> GDLADRFAELERRYDARLGVYVPATGTTAAIEYRADERFAFCSTFKAPLVAAVLHQNPLTHLDKLITYTSDDIRSISPVAQQHVQTGMTIGQLCDAAIRYSDGTAANLLLADLGGPGGGTAAFTGYLRSLGDTVSRLDAEEPELNRNPPGDERDTTTPHAIALVLQQLVLGNALPPDKRALLTDWMARNTTGAKRIRAGFPADWKVIDKTGTGDYGRANDIAV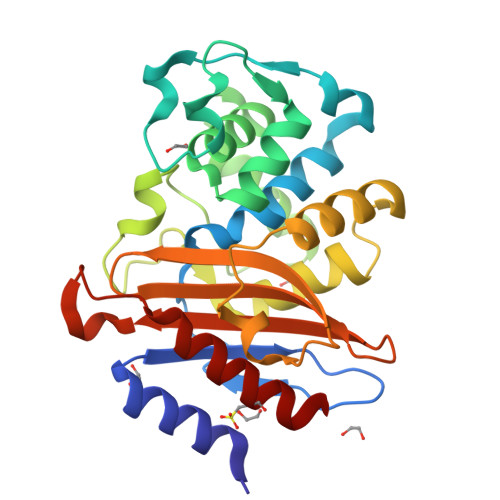VWSPTGVPYVVAVMSDRAGGGYDAEPREALLAEAATCVAGVLA>[3x]SNAMKPIAIYPGTFDPLTNGHVDIIERALPLFNKIIVACAPTSR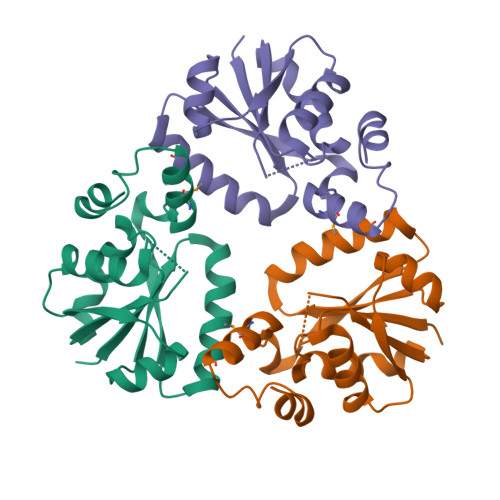KDPHLKLEERVNLIADVLTDERVEVLPLTGLLVDFAKTHQANFILRGLRAVSDFDYEFQLAHMNYQLSPEIETIFLPAREGYSYVSGTMVREIVTLGGDVSPFVPPLVARHLQKRREK> NPCLTGPRTCKDLLDRGHFLSGWHTIYLPDCRPLTVLCDMDTDGGGWTVFQRRVDGSVDFYRDWATYKQGFGSRLGEFWLGNDNIHALTAQGTSELRTDLVDFEDNYQFAKYRSFRVADEAEKYNLVLGAFVEGSAGDSLTFHNNQSFSTKDQDNDLNTGNCAVMFQGAWWYKNCHTSNLNGRYLRGTHGSFANGINWKSGKGYNYSYKVSEMKVRPA;> NPCLTGPRTCKDLLDRGHFLSGWHTIYLPDCRPLTVLCDMDTDGGGWTVFQRRVDGSVDFYRDWATYKQGFGSRLGEFWLGNDNIHALTAQGTSELRTDLVD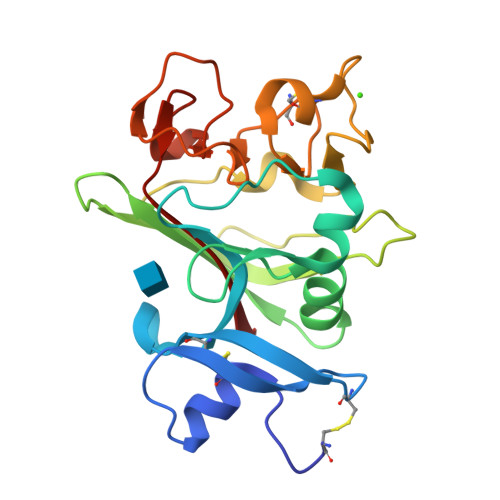FEDNYQFAKYRSFKVADEAEKYNLVLGAFVEGSAGDSLTFHNNQSFSTKDQDNDLNTGNCAVMFQGAWWYKNCHTSNLNGRYLRGTHGSFANGINWKSGKGYNYSYKVSEMKVRPA>SNAMSRGMSGLEDSSDLVVSPYVRMGGLTTDPVPTGGDDPHKVAMLGLTFDDVLLLPAASDVVPATADTSSQLTKKIRLKVPLVSSAMDTVTESRMAIAMARAGGMGVLHRNLPVAEQAGQVEMVKRSGGLLVGAAVGVGGDAWVRAMMLVDAGVDVLVVDTAHAHNRLVLDMVGKLKSEVGDRVEVVGGNVATRSAAAALVDAGADAVKVGVGPGSICTTRVVAGVGAPQITAILEAVAACRPAGVPVIADGGLQYSGDIAKALAAGASTAMLGSLLAGTAEAPGELIFVNGKQYKSYRGMGSLGAMRGRGGATSYSKDRYFADDALS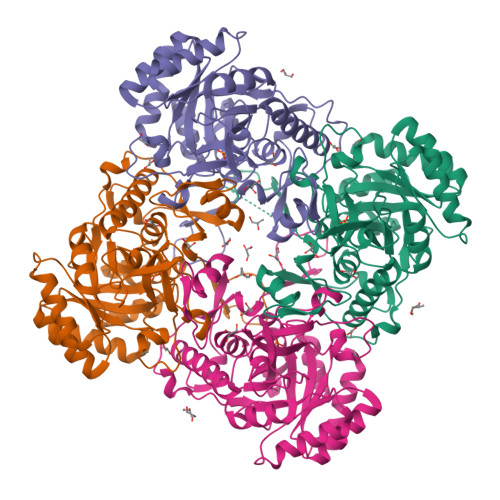EDKLVPEGIEGRVPFRGPLSSVIHQLTGGLRAAMGYTGSPTIEVLQQAQFVRITPAGLKESHPHDVAMTVEAPNYYAR[4x]> AASDWKPGYSMPVLYKYLNSPMERVSLWNYGKPVTLPTGCMMNVAKYTQLCQYLNTTTLAVPVNMRVLHLGAGSEKGVAPGSAVLRQWLPAGTILVDNDLYPFVSDSVATYFGDCITLPFDCQWDLIISDMYDPITKNIGEYNVSKD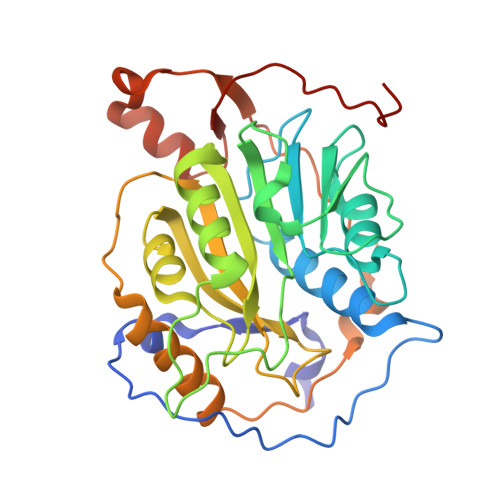GFFTYICHMIRDKLALGGSVAIKITEFSWNAELYKLMGYFAFWTVFCTNANASSSEGFLIGINYLCKPKVEIDGNVMHANYLFWRNSTVWNGGAYSLFDMAKFPLKLAGTAVINLRADQINDMVYSLLEKGKLLIRDTNKEVFVGDSLVNVI> MASMTGGQQMGRDEAGITGTWYNQLGSTFIVTAGADGALTGTYESAVGNAESRYVLTGRYDSAPATDGSGTALGWTVAWKNNYRNAHSATTWSGQYVGGAEARINTQWLLTCGTTEANAWKSTLVGHDTFTKVKPSAASIDAAKKAGVNNGNPLD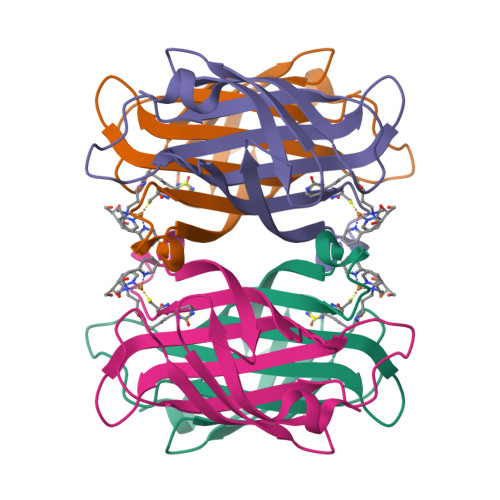AVQQ>MRVKHYIQREFNYSVSSQDLLDIATRIAISAIKPKPKSNKPEPYVDSSTINSLLSFLQSRRNVNELLLYIMRQAGRDEIDEETGKLLLASLKDRELKDAVNLLGYVKWVYDTLTGLKVNYNNVKGVKTFKELVNILSKV[5x];>[2x]MSCMDLDVITTVVKIEGKLRNETLLRVGKGKTQDFAEATDNPIIKYRDRPLIPGSSLKGAFRSLVESYTKSLNDSKYYVCDLDDNSCVSCEEKKKDNGIVEGRYCIPCILFGFKDLASRVYILDAIAEKYSISQRTMVAINRVFGGQMPGHLYTLDYVDPGSEFSFMMMIYNLNLIEGEKDWKAKSVEALKFLLATLVREGIFVGARKSVGYGLIKLVDAKVSLYKAPDHLVSPVIVKKLEEVIGTNG;>MVNYTFIDKRVIKRTTMIEGDVETVSPLKIGGGKDNFDPSSLAKDSILKDVEGRPIIPGSSWKGIFRSTGERILRLRNIEVCSGIGKDYCLNNNRKERDFNSALKENVDQALEIFWDYTCLNCKVFGTMSVIGAVRFLDSLPISYSLNTRSMIAISRTEGAVARRALVTVEYVDVGSKFSFKMMGYNLPNYAIGYLITIMKNIHDGFTQVGGHKSRGFGFVKFGKVKFTDLGEKRIGDEDIQVKDVGDLVEGNGDEFFGRMKPFMEAFNNAKIPYPKK[2x];> RSPIRRSNYTPRNEKGLEGVIELQLNVVSDYLHVGSGKYDVEVMRSVSDVKRLVEDYLSGGNKRIPNNVDQYFSMVAFLMVRNKDNVVIPGSTIKGMVRSRLELSVPGSCYIVTGHSTSSSAVYKRIFNPDPNRGSDRFDVNKFPQVCPVCDLLGNMGLASRVSLSDFVMTSGKVDYVNVKGRDYEVVTKGSIFAGKVLYKSLKPVEIGMLLYGFGFVKDCNGSKVMLLGRFKFSDKRFGRVKFSLKTPIADCNKLVSDFVKQFNPRYINEE;> MIRGKLLLPEKKVVFINESEVQSLRKDVVDALKVFSSLACELADNNETKATNIFADLISMIYKLPMLISYVPSDKLSTPHEYFFAYIVFRHLVEDSMPSNDIAKLLEILEEKKRDEIKEVLDYARTLRKIYEKLLYVPADTRPGYNFTSLASHLQLSSILVWLLQKGSVDLNYLRISALLHDIGKLFNPTNHVSESIKILDEVIEGSECLKTNLSRVKSLVEQHHAPLETILNDADRLAASTDRFSEIVKGALNNTKIGECYSLCYGRDVRTKECMECLEEYGEETYSEESKRLYDVISNSVVSQKVEGNAIGYLVYIDFPGIQRFITSFPKLREMSFASFLVDFVTSIYSFIVLDQAYYERTGKKSRIPAEALLSGYGGHSYIIVRSDFGSKDEVKAWLESVSSSALSKLGIRLDVKVADFAYENYVRNYKEVYEDMMSKSYERYLIRDEGKVYSYGLHRVCDNCGIRPAVNRSDDGEYLCETCNLVRDLSKNRGFIAKYKSKYTLYEEQRIEISPKEDIKFKLDKNQDPTSYAMEIIAGYRTTSDSRYIALIKADGNNAGKIFGNTVTFSEYVDKSFRLDFGVKKMFYDTLLDIMRASSDESIKKDLVSRILLGVLYLGGDDIMLLSPSAIAVPFAVKMFKRSLEYTGFTFKVGIISVKPDHPVQFAYGAVNALMEESKIHTGEKSSIGVLVFSSTLASEGVVKSDLKNYRKEKESFLVVSNDVDDVERLLNLMELDDFGKLMELYWNPEEGRKVIRDKIRSLERFVNYADTHDFYNTLAYLIRSKAKSEENSLIKRIIDLTIKGRDDFVFPLYDYYFILKSIRVGI;> MIPIKVSMRNLSSLTIAGGSTISSIDIPLNPLGVPPSTIKGTMRTAVHNLLPNGYTSCGEVEPESIREAHKNGVCDVCKLFGYPDSLTGCFTIDVSKTDYRTSYITRVSIDDKTQRAKEGSLFTQQIILPNSDISFTVYYNCNDERLFKLLLYSILDLRYWRLGRNTMIDVKVNNVEEICKSVKCDEEINGILNQLSRYLWE;> MILIKLKVKGYITTQMRRIRNYYFSITNYIPSTTLRGAILAEYYNQTGKIDENFYVSPAYPIKTAPAHYFSPAKERKGDEFIEVKRILEKKEKEFEANKPIEEIMKLEIDGKHPKPKIGSLITYEGETDKENKYREFSSKSIIQMHVAIDKTSISSYKGMLFAYEYKEFDEMWAIASDSEVIDTVKRIKIGRGKNRGNKVVDVEKVREVSLDQSKGLLYCLSPCIGSLFGKTFFKAKYIIGDKSIYSGWFTVDSFSGQKPVFETLREGSLVYVESFSNEKSLMPAGLNFMLRISDLSSIL;> MVIQVFRLNFRLRTGFRVGGGQEVGDNVIRQLRIGVEGVMIPA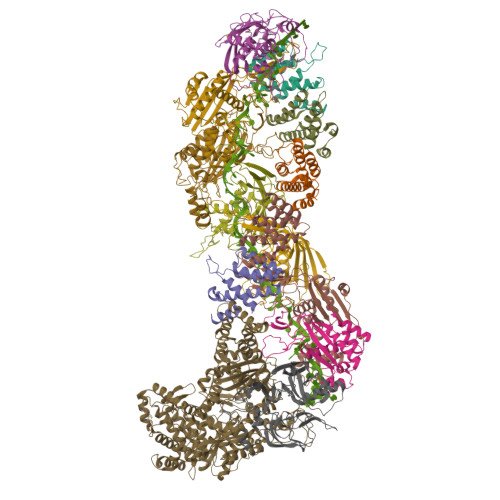SSWKGMFRRVSEIVLNSEDHFEEHSKKEVDTRTINALLKSDEKFRRIAISKVGKEVITQNGINVDKLDSESLSDLRRIYNEYNCPIERLYGSNYFAGGITISDSVIPNASIMERTHVTIERKSKKASEKHLFSEEIIDAEKIEVKVIVRNEFELWKNSLKLLREIGYFIGGSKSRGIGYIVLDEKESEYAVINNFSETPKFSELKRYLS Within their active site, molybdenum or tungsten are chelated by a metal-binding pterin (MPT, also known as molybdopterin) forming the so-called molybdenum (Moco) or tungsten cofactors (Wco), respectively. Wco and Moco biosyntheses represent multistep pathways that start from GTP and involve three isolatable intermediates: cyclic pyranopterin monophosphate (cPMP), MPT and adenylylated MPT (MPT-AMP). MPT-adenylyl-transferases (EC 2.7.7.75) convert MPT to MPT-AMP, prior to the final metal insertion step, which requires either tungstate or molybdate to produce Wco and Moco, respectively. In this study we investigated the influence of hexamerization on the structural stability and enzymatic activity of P. furiosus MPT-adenylyl-transferase MoaB (PfuMoaB).

We determined the crystal structure of PfuMoaB at 2.5 Å resolution and engineered a hexamerization-deficient variant of PfuMoaB using structure-guided mutagenesis. PfuMoaB was crystallized in the space group P3121 with three molecules (chains A, B and C) in the asymmetric unit. Each PfuMoaB subunit consists of a slightly bent central β-sheet, surrounded by six α-helices and two 310 helices. In the crystal structure a hexamer can be generated by rotation of the asymmetric unit by 180° around the two-fold crystallographic symmetry axis. Therefore, similar to the other proteins of the MoaB family, PfuMoaB represents a dimer of trimers. In the crystal structure of PfuMoaB residual electron density was observed in close proximity to the Gly-Gly-Thr-Gly motif. PfuMoaB crystals were grown in a solution containing 2-(N-morpholino)ethanesulfonic acid (MES), which with its negatively charged sulfonate part resembles sulfate or phosphate. Therefore, only a sulfate molecule was manually positioned into the respective electron density patch leading to an improved overall model quality. Assembly of subunits into trimers is additionally strengthened through several ionic interactions, including salt bridges between Arg109 of one monomer and Glu106 of another monomer, and a cluster of ionic interactions involving Lys100 of one subunit and Arg124 and Glu92 of the adjacent polypeptide chain. Thus, hydrophobic residues of α3-helix were identified as key residues for the association of two trimers within the hexamer.

>HHHHHHSSGLVPRGSHMMGVEEHKKEAPKTFKFGVITVSDKGAKGEREDKSGPLIIEELSKLGEHVYYKIVPDDKIEVLIALFEAIKSGADVVVTTGGTGITRRDITIESIKPLFDKELSFGEVFRAKSYEEVGYATVLTRATAGIIRGQERIVVVFSLPGSVNAVKTGLEIIKSEVFHILKHARE[3x]> APMGSDPPTACCFSYTARKLPRNF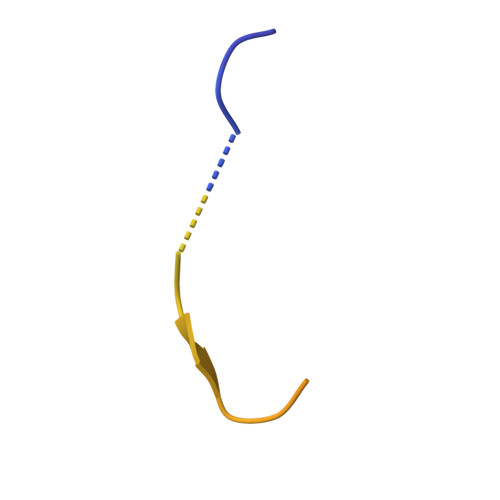VVDYYETSSLCSQPAVVFQTKRSKQVCADPSESWVQEYVYDLELN4-[(1S,4S)-5-(3-chlorophenyl)-2,5-diazabicyclo[2.2.1]heptan-2-yl]-2-(pyridin-3-yl)pyrimidine-5-carbonitrile 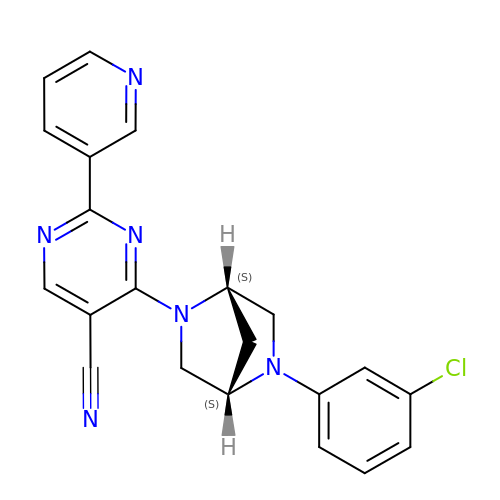| C21 H17 Cl N6 | LYMCCCUAFBZMES-OALUTQOASA-N> ATFEIVNRCSYTVWAAASKGDAALDAGGRQLNSGESWTINVEPGTNGGKIWARTDCYFDDSGSGICKTGDCGGLLRCKRFGRPPTTLAEFSLNQYGKDYIDISNIAGFNVPMDFSPTTRGCRGVRCAADIVGQCPAKLKAPGGGCNDACTVFQTSEYCCTTGKCGPTEYSRFFKRLCPDAFSYVLDKPTTVTCPGSSNYRVTFCPTA

Among the sweet-tasting proteins, thaumatin is ~100,000 times sweeter than sucrose on a molar basis and about 1,600 times sweeter on a weight basis. The intensely sweet taste of thaumatin has been widely used not only as a natural sweetener, but also as a flavor enhancer and for masking unpleasant tastes in the food and pharmaceutical industries. Site-directed mutagenesis studies revealed that six lysine residues of Lys19, Lys49, Lys67, Lys106, Lys163, and Lys187, and three arginine residues of Arg76, Arg79, and Arg82 located on the cleft-containing side are responsible for sweetness, and two amino acids residues, Lys67 and Arg82, are particularly important for sweetness. In the present study, three mutant X-ray crystallographic structures of thaumatin (K78A, K106A, and K137A) were determined at resolutions of 1.07, 1.07 and 1.01 Å, respectively.

The threshold values of sweetness of K49A, K106A, and K163A were 140, 140, and 180 nM, respectively, which is about a 3.1- to 4-fold reduction of sweetness. The structure consists of 3,267 protein atoms including hydrogen atoms, 20 tartrate atoms, 18 glycerol atoms and 300 water molecules. The normalized B-factor ratio of Ala106 was 0.68 for main-chain and 0.72 for side-chain and those of Lys106 in recombinant thaumatin for main-chain and side-chain were 0.61 and 1.25, respectively. The normalized B-factor ratio decreased by 0.53 for side-chain, suggesting that the flexibility of side-chain was also reduced. Besides, the flexibility of Lys106 is substantially lower than that of Lys78 and Lys137 in wild type structure, suggesting that the lower flexibility of side-chain at interaction sites might not help support good complementarity with sweet receptor. The detailed structural assignment at an atomic level revealed no significant conformational changes in interaction sites of Ala106 as well as Arg82 were induced by mutation. With K106A thaumatin, the volume of positive charge from lysine residue was reduced but the distribution of charge was relatively small when compared to K78A and K137A. Compared to Lys78 and Lys137, Lys106 is not relatively exposed to the molecular surface. As to Lys106, it was 5.0 Å from CG of Asp173_T1R2, which also interacted with Arg82 in the length of 4.6 Å. Since the interaction to Asp173_T1R2 still is retained, substantial reduction of sweetness might not be induced by K106A.> MVLGKVVGTVVASRKEPRIEGLSLLLVRACDPDGTPTGGAVVCADAVGAGVGEVVLYASGSSARQTEVTNNRPVDATIMAIVDLVEMG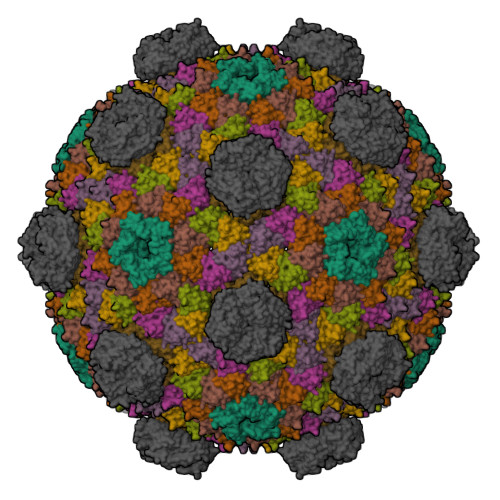GDVRFRKD;>[6x]MADALGMIEVRGFVGMVEAADAMVKAAKVELIGYEKTGGGYVTAVVRGDVAAVKAATEAGQRAAERVGEVVAVHVIPRPHVNVDAALPLGRTPGMDKSA;>[2x]MSITLRTYIFLDALQPQLATFIGKTARGFLPVPGQASLWVEIAPGIAINRVTDAALKATKVQPAVQVVERAYGLLEVHHFDQGEVLAAGSTILDKLEVREEGRLKPQVMTHQIIRAVEAYQTQIINRNSQGMMILPGESLFILETQPAGYAVLAANEAEKAANVHLVNVTPYGAFGRLYLAGSEAEIDAAAEAAEAAIRSVSGVAQESFRDR>[6x]MKWFNTLSHNRWLEQETDRIFNFGKNAVVPTGFGWLGNKGQIKEEMGTHLWITARMLHVYSVAASMGRPGAYDLVDHGIKAMNGALRDKKYGGWYACVNDQGVVDASKQGYQHFFALLGAASAVTTGHPEARKLLDYTIEVIEKYFWSEEEQMCLESWDEAFSQTEDYRGGN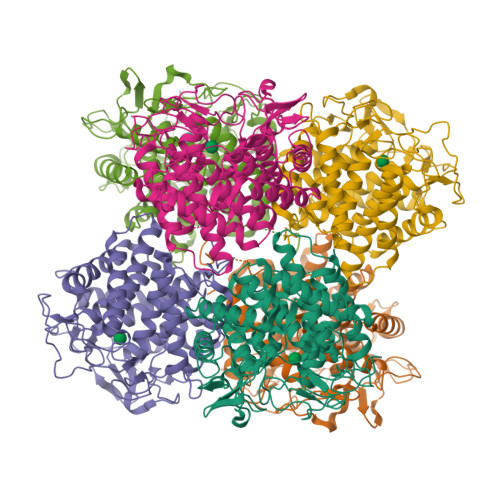ANMHAVEAFLIVYDVTHDKKWLDRALRIASVIIHDVARNGDYRVNEHFDSQWNPIRDYNKDNPAHRFRAYGGTPGAWIEWGRLMLHLHAALEARFETPPAWLLEDAKGLFHATIRDAWAPDGADGFVYSVDWDGKPIVRERVRWPIVEAMGTAYALYTLTDDSQYEEWYQKWWDYCIKYLMDYENGSWWQELDADNKVTTKVWDGKQDIYHLLHCLVIPRLPLAPGLAPAVAAGLLDINAKLEHHHHHH3-[(4-CHLOROANILINO)SULFONYL]THIOPHENE-2-CARBOXYLIC 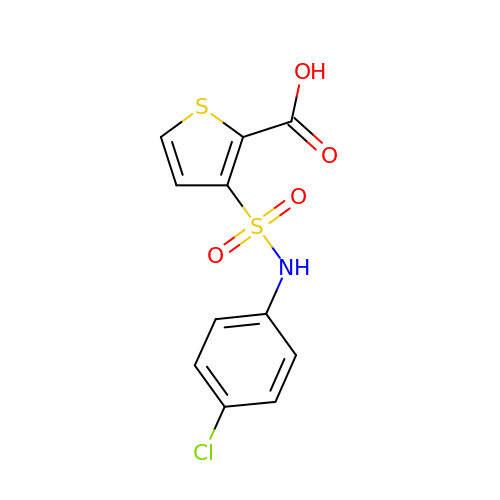ACID | C11 H8 Cl N O4 S2 | YRWKEEDITQJPCZ-UHFFFAOYSA-N> MHHHHHHAAGIPMNNPAIKRIGNHITKSPEDKREYRGLELANGIKVLLISDPTTDKSSAALDVHIGSLSDPPNIAGLSHFLQHMLFLGTKKYPKENEYSQFLSEHAGSSNAFTSGEHTNYYFDVSHEHLEGALDRFAQFFLSPLFDESAKDREVNAVDSEHEKNVMNDAWRLFQLEKATGNPKHPFSKFGTGNKYTLETRPNQEGIDVRQELLKFHSAYYSSNLMAVVVLGRESLDDLTNLVVKLFSEVENKNVPLPEFPEHPFQEEHLKQLYKIVPIKDIRNLYVTFPIPDLQKYYKSNPGHYLGHLIGHEGPGSLLSELKSKGWVNTLVGGQKAGARGFMFFIINVDLTEEGLLHVEDIILHMFQYIQKLRAEGPQEWVFQELKDLNAVAFRFKDKERPRGYTSKIAGILHYYPLEEVLTAEYLLEEFRPDLIEMVLDKLRPENVRVAIVSKSFEGKTDRTEEWY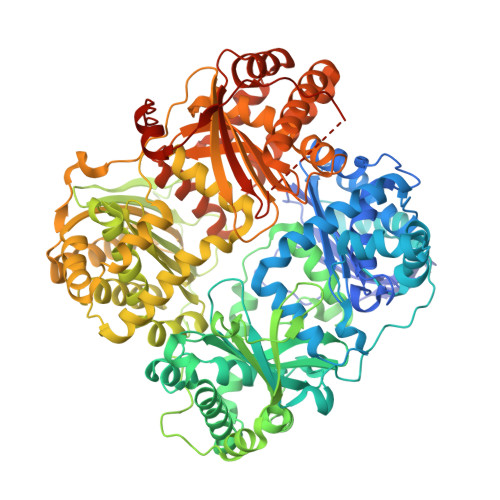GTQYKQEAIPDAVIAKWQNAALNGKFKLPTKNEFIPTNFEILPLEAAATPYPALIKDTAMSKLWFKQDDKFFLPKANLNFEFFSPFAYVDPLHSNMAYLYLELLKDSLNEYAYAAELAGLSYDLQNTIYGMYLSVKGYNDKQPILLKKIIEKMATFEIDEARFEIIKEAYMRSLNNFRAEQPHQHAMYYLRLLMTEVAWTKDELKEALADVTLPRLKAFIPQLLSRLHIEALLHGNITKQAALGIMQMVEDTLIEHAHTKPLLPSQLAAYREVQLPDRGWFVYQQRNEVHNNSGIEIYYQTDMQSTSENMFLELFAQIISEPAFNTLRTKEQLGYIVFSGPRRANGIQGLRFIIQSEKPPHYLESRVEAFLITMEKSIEDMTEEAFQKHIQALAIRRLDKPKKLSAESAKYWGEIISQQYNFDRDNTEVAYLKTLTKADIIKFYKEMLAVDAPRRHKVSVHVLAREMDSNPVVGEFPAQNDINLSQAPALPQPEVIQNMTAFKRGLPLFPLVKPHINFMAAKL>[2x]GSHMKFTRVCDRRDVPEGEALKVESGGTSVAIFNVDGE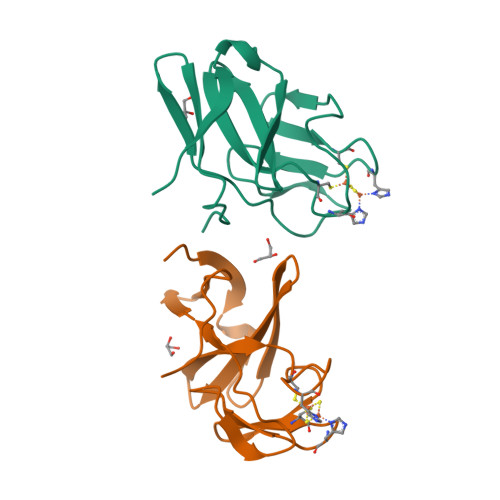LFATQDRCTHGDWSLSDGGYLEGDVVECSLHMGKFCVRTGKVKSPPPCEALKIFPIRIEDNDVLVDFEAGYLAP> MAEILRAENIKKVIRGYEILKGISLSVKKGEFVSIIGASGSGKSTLLYILGLLDAPTEGKVFLEGKEVDYTNEKELSLLRNRKLGFVFQFHYLIPELTALENVIVPMLKMGKPKKEAKERGEYLLSELGLGDKLSRKPYELSGGEQQRVAIARALANEPILLFADEPTGNLDSANTKRVMDIFLKINEGGTSIVMVTHERELAELTHRTLEMKDGKVVGE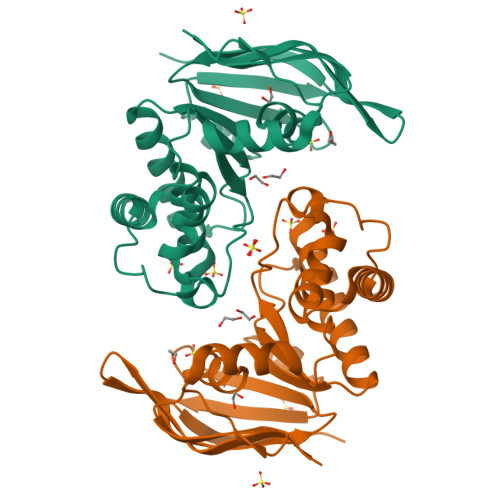ITRV> SAGAGSHCQKTSLRVNFEDIGWDSW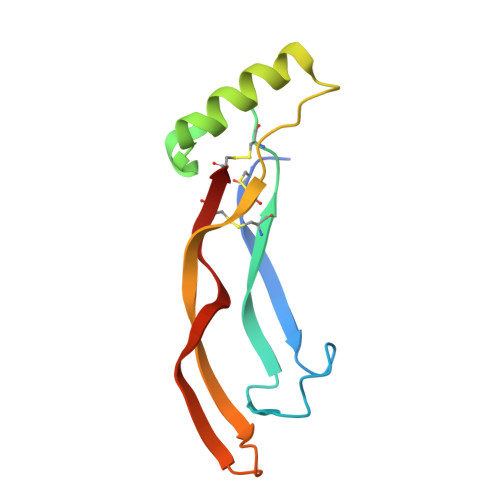IIAPKEYEAYECKGGCFFPLADDVTPTKHAIVQTLVHLKFPTKVGKACCVPTKLSPISVLYKDDMGVPTLKYHYEGMSVAECGCR>GSTSSLDKYLTESQFHDKRIAEELRT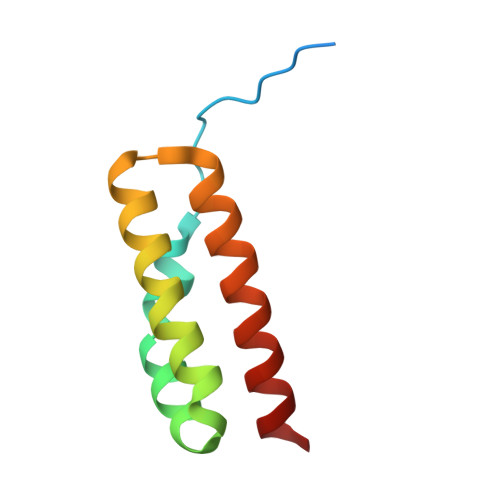LLNKSNVYALAAGSLNPYYKRTIMMNEYRAKAALKKNDFVSMADAKVALEKIYKEIDEIINR[3x]>[2x]PISPIETVPVKLKPGMDGPKVKQWPL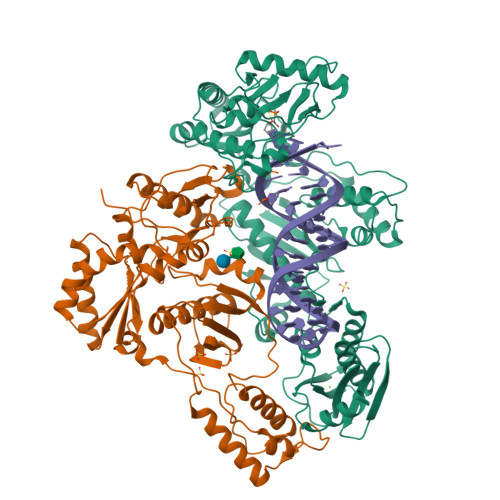TEEKIKALVEICTEMEKEGKISKIGPENPYNTPVFAIKKKDSTKWRKLVDFRELNKRTQDFWEVQLGIPHPAGLKKKKSVTVLDVGDAYFSVPLDEDFRKYTAFTIPSINNETPGIRYQYNVLPQGWKGSPAIFQSSMTKILEPFKKQNPDIVIYQYMDDLYVGSDLEIGQHRTKIEELRQHLLRWGLTTPDKKHQKEPPFLWMGYELHPDKWTVQPIVLPEKDSWTVNDIQKLVGKLNWASQIYPGIKVRQLSKLLRGTKALTEVIPLTEEAELELAENREILKEPVHGVYYDPSKDLIAEIQKQGQGQWTYQIYQEPFKNLKTGKYARMRGAHTNDVKQLTEAVQKITTESIVIWGKTPKFKLPIQKETWETWWTEYWQATWIPEWEFVNTPPLVKLWYQLEKEPIVGAETFYVDGAANRETKLGKAGYVTNKGRQKVVPLTNTTNQKTELQAIYLALQDSGLEVNIVTDSQYALGIIQAQPDKSESELVNQIIEQLIKKEKVYLAWVPAHKGIGGNEQVDKLVSAG;>[2x]MAHHHHHHALEVLFQGPISPIETVPVKLKPGMDGPKVKQWPLTEEKIKALVEICTEMEKEGKISKIGPENPYNTPVFAIKKKDSTKWRKLVDFRELNKRTQDFWEVQLGIPHPAGLKKKKSVTVLDVGDAYFSVPLDEDFRKYTAFTIPSINNETPGIRYQYNVLPQGWKGSPAIFQSSMTKILEPFKKQNPDIVIYQYMDDLYVGSDLEIGQHRTKIEELRQHLLRWGLTTPDKKHQKEPPFLWMGYELHPDKWTVQPIVLPEKDSWTVNDIQKLVGKLNWASQIYPGIKVRQLSKLLRGTKALTEVIPLTEEAELELAENREILKEPVHGVYYDPSKDLIAEIQKQGQGQWTYQIYQEPFKNLKTGKYARMRGAHTNDVKQLTEAVQKITTESIVIWGKTPKFKLPIQKETWETWWTEYWQATWIPEWEFVNTPPLVKLWYQ>[24x]EEAELAYLLGELAYKLGEYRIAIRAYRIALKRDPNNAEAWYNLGNAYTKQGDYDEAIEYYLRALVLDPNNAEAATNLGQAYMNQGDKDRAKLMLLLALKLDPNNDSARVILGVAKVGIEELAKLASQAQQEGDSEKQKAIELAAEAARVAQEVGDPELEK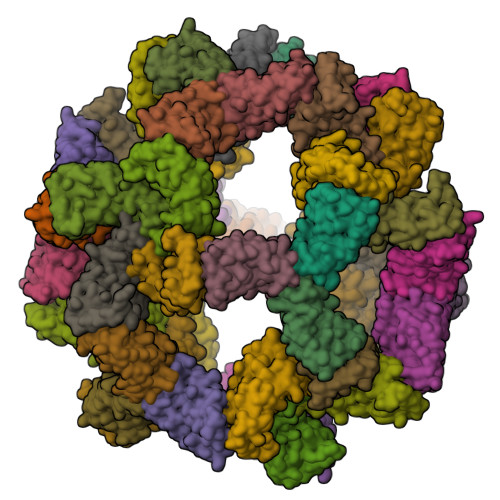LALEAARRGDSEKAKAILLAAEAARVAKEVGDPELIKLALEAARRGDSEKARAILEAAERAREAKERGDPEQIKKARELAKR;>[24x]DVSALAYVMLGLLLSLLNRLSLAAEAYKKAIELDPNDALAWLLLGSVLEKLKRLDEAAEAYKKAIELKPNDASAWKELGKVLEKLGRLDEAAEAYLIAIMLDPEDAEAAKELGKVLEKLGELEMAEEAYKLAIKLDPND> GSHMTDLLASTLEHLETLVSFDTRNPPRAIAAEGGIFDYLRAQLPGFQVEVIDHGDGAVSLYAVRGTPKYLFNVHLDTVPDSPHWSADPHVMRRTEDRVIGLGVCDIKGAAAALVAAAN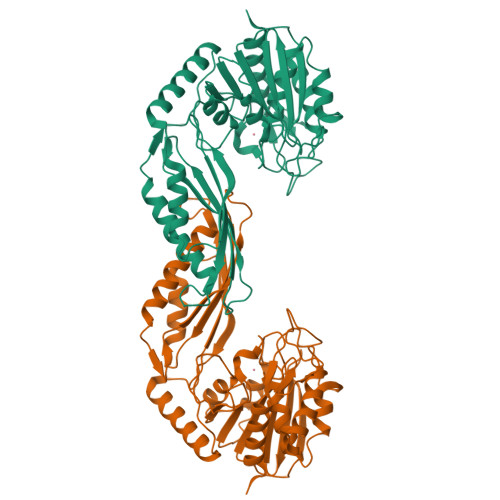AGDGDAAFLFSSDEEANDPRCIAAFLARGLPYDAVLVAEPTMSEAVLAHRGISSVLMRFAGRAGHASGKQDPAASALHQAMRWGGKALDHVESLAHARFGGLTGLRFNIGRVDGGIKANMIAPAAELRFGFRPLPSMDVDGLLATFAGFADPAAAHFEETFRGPSLPSGDIARAEERRLAARDVADALDLPIGNAVDFWTEASLFSAGGYTALVYGPGDIAQAHTADEFVTLAQLQRYVESVNRIINGSH> MIVSAIAANALLESVTKFHCGVIYDYSTAEYVSYRPSDFGAYLDALEAEVARGGLIVFHNGHKYDVPALTKLAKLQLNREFHLPRENCIDTLVLSRLIHSNLKDTDMGLLRSGKLPGKRFGSHALEAWGYRLGEMKGEYKDDFKRMLEEQGEEYVDGMEWWNFNEEMMDYNVQDVVVTKALLEKLLSDKHYFPPEIDFTDVGYTTFWSESLEAVDIEHRAAWLLAKQERNGFPFDTKAIEELYVELAARRSELLRKLTETFGSWYQPKGGTEMFCHPRTGKPLPKYPRIKTPKVGGIFKKPKNKAQREGREPCELDTREYVAGAPYTPVEHVVFNPSSRD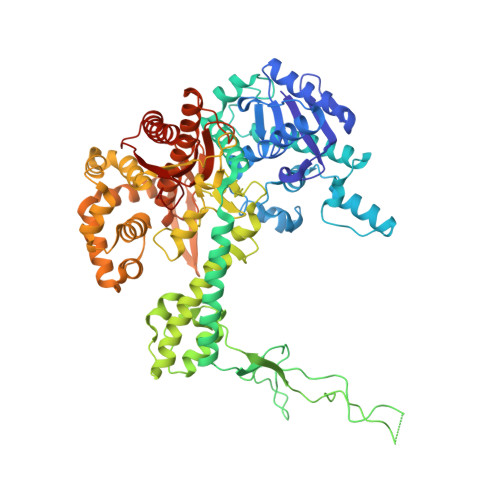HIQKKLQEAGWVPTKYTDKGAPVVDDEVLEGVRVDDPEKQAAIDLIKEYLMIQKRIGQSAEGDKAWLRYVAEDGKIHGSVNPNGAVTGRATHAFPNLAQIPGVRSPYGEQCRAAFGAEHHLDGITGKPWVQAGIDASGLELRCLAHFMARFDNGEYAHEILNGDIHTKNQIAAELPTRDNAKTFIYGFLYGAGDEKIGQIVGAGKERGKELKKKFLENTPAIAALRESIQQTLVESSQWVAGEQQVKWKRRWIKGLDGRKVHVRSPHAALNTLLQSAGALICKLWIIKTEEMLVEKGLKHGWDGDFAYMAWVHDEIQVGCRTEEIAQVVIETAQEAMRWVGDHWNFRCLLDTEGKMGPNWAICH> VILPNNDRHQITDTTNGHYAPVTYIQVEAPTGTFIASGVVVGKDTLLTNKHVVDATHGDPHALKAFPSAINQDNYPNGGFTAEQITKYSGEGDLAIVKFSPNEQNKHIGEVVKPATMSNNAETQTNQNITVTGYPGDKPVATMWESKGKITYLKGEAMQYDLSTTGGNSGSPVFNEKNEVIGIHWGGVPNEFNGAVFINENVRNFLKQNIEDINFANDDQPNNPDNPDNPNNPDNPNNPDN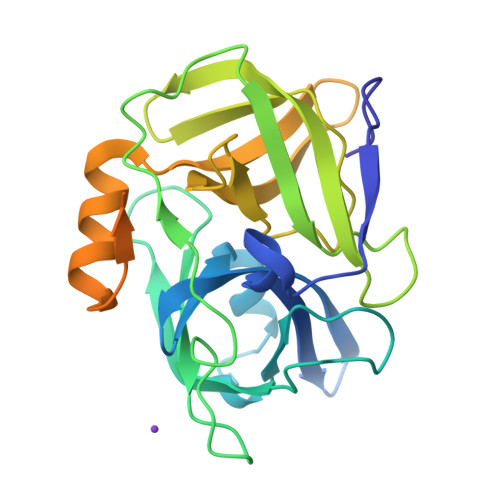PNNPDEPNNPDNPNNPDNPDNGDNNNSDNPDAA>MNDEAPVFTQQQYNRLGLRETAGIGTSVIVVRATDKDTGDGGLVNYRILSGAEGKFEIDESTGLIVTVDYLDYETKTSYLMNVSATDGAPPFNQGFCSVYVTLLNELDEAVQFSNASYEAVIMENLALGTEIVRVQAYDIDNLNQITYRFDAYTSAQAKALFKIDAITGVITV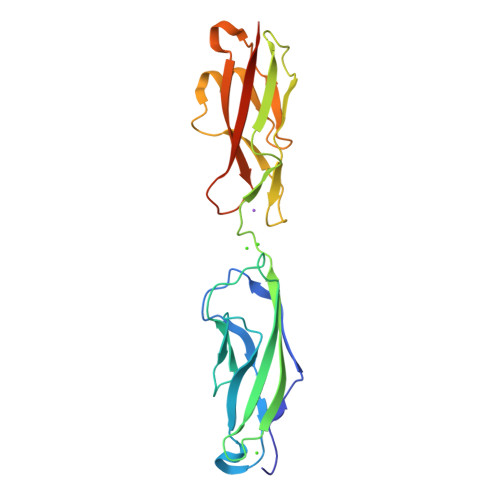KGLVDREKGDFYTLTVVADDGGPKVDSTVKVYITVLDENLEHHHHHH[4x]3-(4-AMINO-2-TRIFLUOROMETHYL-PYRIMIDIN-5-YLMETHYL)-4-METHYL-5-(2-PHOSPHONATOOXY-ETHYL)-THIAZOL-3-IUM | C12 H13 F3 N4 O4 P S | 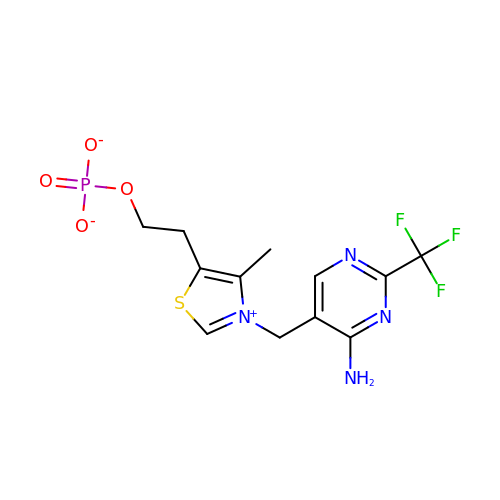ZIBIECXVPMYJCV-UHFFFAOYSA-M Fms-like tyrosine kinase 3 (FLT3) is a member of the class III family of receptor tyrosine kinases expressed on early hematopoietic stem and progenitor cells, and plays an important role in hematopoiesis. Wild-type FLT3 (FLT3wt) is activated by FLT3 ligand (FL), which promotes receptor dimerization, auto-phosphorylation, and cell proliferation via activation of its downstream signaling molecules, including STAT5, ERK1/2, and AKT. FLT3 is made up of 5 functional domains: an immunoglobulin-like extracellular domain, a transmembrane domain, a juxtamembrane domain (JMD), a tyrosine kinase domain (TKD), and a small C-terminal domain. Mutations at the JMD or TKD of FLT3 induce constitutive kinase activation that is independent of FL, and occurs in approximately one-third of acute myeloid leukemia (AML) patients.

Gilteritinib is a selective FLT3 inhibitor that inhibits both FLT3-ITD and FLT3-TKD mutations, and is classified as an ATP-competitive type I inhibitor. To reveal the binding mode, we determined the crystal structure of the FLT3 kinase domain in complex with gilteritinib. As expected from the computational modeling performed in our previous report, gilteritinib bound to the ATP pocket of FLT3. While the JMD was clearly observed in the overall structure, a portion of the activation loop including Gly831 in the DFG motif was disordered. Asp829 and Phe830 in the DFG motif adopted the “DFG-out” conformation. In the binding mode of gilteritinib, two hydrogen bonds were formed between the carbamoyl group and the main chain atoms of Glu692 and Cys694. There was no distinct interaction between gilteritinib and the activation loop including Asp829 and Phe830. The crystal structure of the complex formed between FLT3 and gilteritinib was obtained using the kinase domain of FLT3wt, including the JMD, which has been reported to bind to the active site of FLT3 and to stabilize the autoinhibited form. In the complex structure with gilteritinib, the JMD bound to the active site, indicating that FLT3 adopted the autoinhibited form. Gilteritinib was far from the active conformation of the activation loop, suggesting that it likely binds to the active form of FLT3 as well as the autoinhibited form.

> RYESQLQMVQVTGSSDNEYFYVDFREYEYDLKWEFPRENLEFGKVLGSGAFGKVMNATAYGISKTGVSIQVAVKMLKEKADSSEREALMSELKMMTQLGSHENIVNLLGACTLSGPIYLIFEYCCYGDLLNYLRSKREKFSEDEIEYENQKRLEEEEDLNVLTFEDLLCFAYQVAKGMEFLEFKSCVHRDLAARNVLVTHGKVVKICDFGLARDIMSDSNYVVRGNARLPVKWMAPESLFEGIYTIKSDVWSYGILLWEIFSLGVNPYPGIPVDANFYKLIQNGFKMDQPFYATEEIYIIMQSCWAFDSRKRPSFPNLTSFLGCQLADAE N,N'-bis[3-(4,5-dihydro-1H-imidazol-2-yl)phenyl]biphenyl-4,4'-dicarboxamide | C32 H28 N6 O2 | 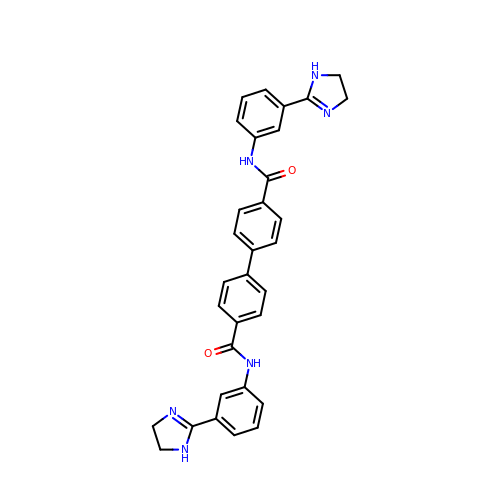HOYOJUMMRGKESB-UHFFFAOYSA-N>[2x]MQNITQSWFVQGMIKATTDAWLKGWDERNGGNLT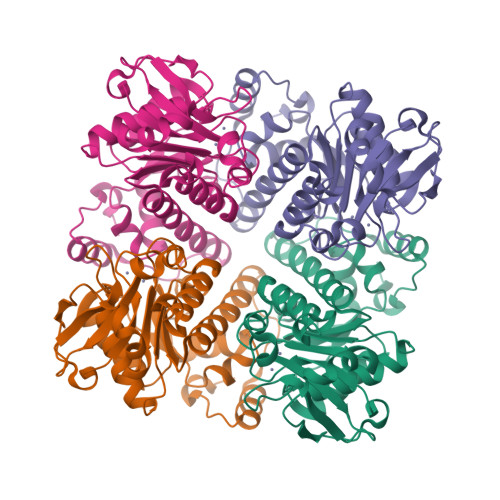LRLDDADIAPYHDNFHQQPRYIPLSQPMPLLANTPFIVTGSGKFFRNVQLDPMANLGIVKVDSDGAGYHILWGLFNEAVPTSELPAHFLSHCERIKATNGKDRVIMHCHATNLIALTYVLENDTAVFTRQLWEGSTECLVVFPDGVGILPWMVPGTDAIGQATAQEMQKHSLVLWPFHGVFGSGPTLDETFGLIDTAEKSAQVLVKVYSMGGMKQTISREELIALGKRFGVTPLASALAL>[6x]GSSGVRLWATRQAMLGQVHEV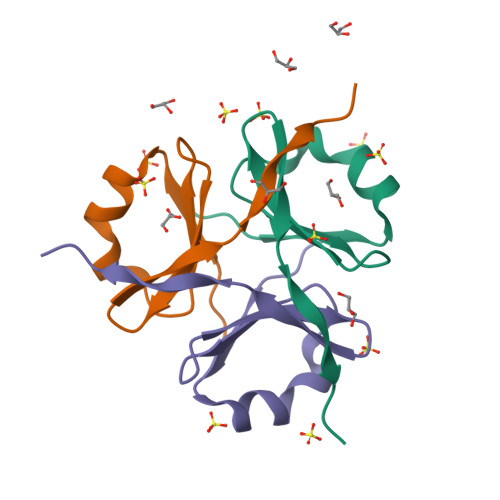PEGWLIFVAEQEELYVRVQNGFRKVQLEARTPLPR> SMDDSETGFNLKVVLVSFKQCLDEKEEVLLDPYIASWKGLVRFLNSLGTIFSFISKDVVSKLRIMERLRGGPQSEHYRSLQAMVAHELSNRLVDLERRSHHPESGCRTVLRLHRALHWLQLFLEGLRTSPEDARTSALCADSYNASLAAYHP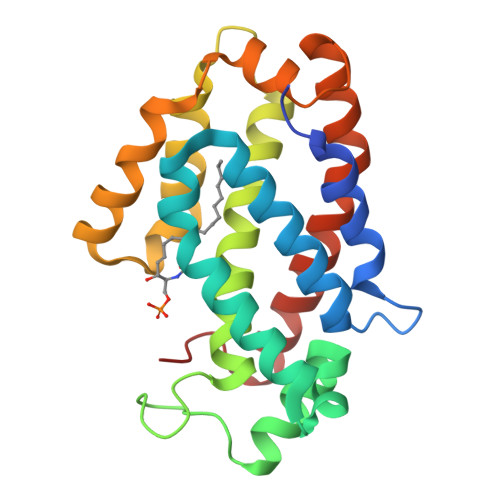WVVRRAVTVAFCTLPTREVFLEAMNVGPPEQAVQMLGEALPFIQRVYNVSQKLYAEHSLLDLP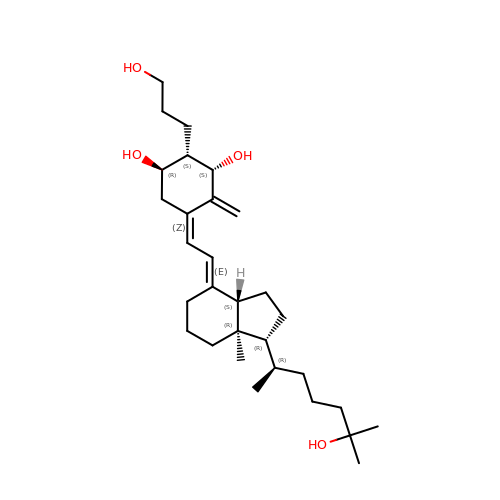2ALPHA-(3-HYDROXYPROPYL)-1ALPHA,25-DIHYDROXYVITAMIN D3 | C30 H50 O4 | QOVWEUHJARWCDV-RQSRSJTKSA-N>SGAKPGKKTRGRVKIKMEFIDNKLRRYTTFSKRKTGIMKKAYELSTLTGTQVLLLVASETGHVYTFATRKLQPMITSETGKALIQTCLNSPD[4x];>[2x]GSDSA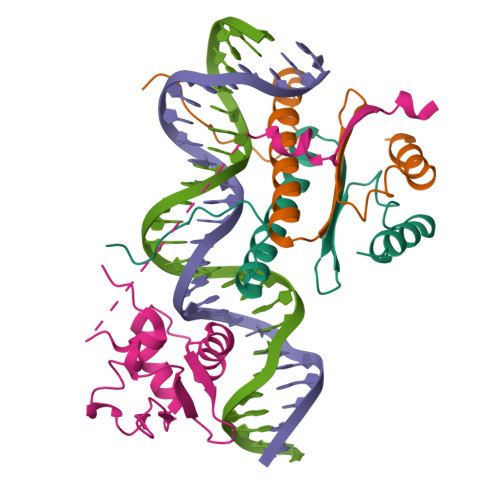ITLWQFLLQLLQKPQNKHMICWTSNDGQFKLLQAEEVARLWGIRKNKPNMNYDKLSRALRYYYVKNIIKKVNGQKFVYKFVSYPEILNMDPMTVGRIEGDCESLNFSEVSSSSKDVENGGKDKPPQPGAKTSSRNDYIHSGLYSSFTLNSLN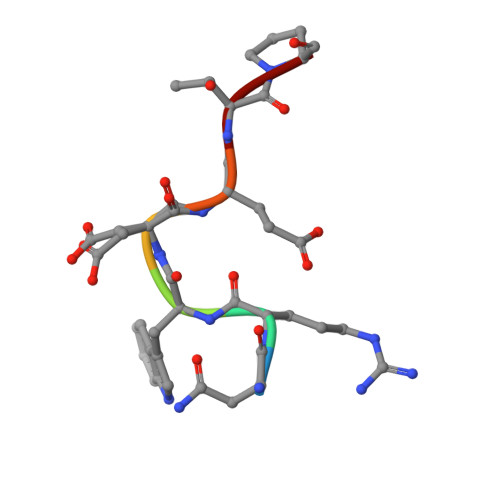> NRWDETP> MYNDDYIEEASFLNGSDVVILIDGV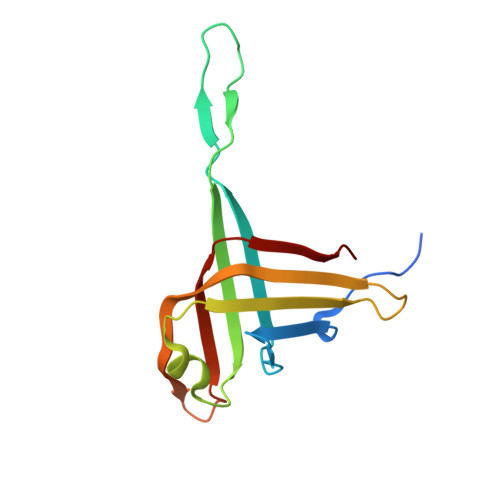EELYMEEIKADFEQDEQSIKLLGCQNEISRVGTTKGSFSLNGYKTDSKFAKLGFRSFEIIYNLSNSETLGYESIRLKNCRLKKLPLINSKAGEIVKIEVEGSFRGYDLLNEL> MASMTGGQQMGRGSMIFSVDKVRADFPVLSREVNGLPLAYLDSAASAQKPSQVIDAEAEFYRHGYAAVHRGIHTLSAQATEKMENVRKRASLFINARSAEELVFVRGTTEGINLVANSWGNSNVRAGDNIIISQMEHHANIVPWQMLCARVGAELRVIPLNPDGTLQLETLPTLFDEKTRLLAITHVSNVLGTENPLAEMITLAHQHGAKVLVDGAQAVMHHPVDVQALDCDFYVFSGHKLYGPTGIGILYVKEALLQEMPPWAGGGSMIATVSLSEGTTWTKAPWRFEAGTPNTGGIIGLGAALEYVSALGLNNIAEYEQNLMHYALSQLESVPDLTLYGPQNRLGVIAFNLGKHHAYDVGSFLDNYGIAVRTGHHCAMPLMAYYNVPAMCR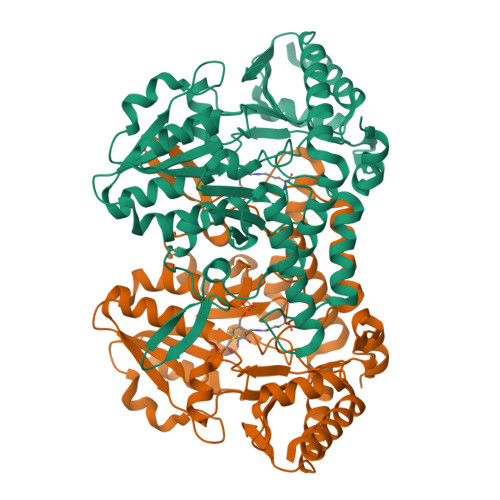ASLAMYNTHEEVDRLVTGLQRIHRLLG> MPGPLGLLCFLALGLLGSAGPSGAAPPLCAAPCSCDGDRRVDCSGKGLTAVPEGLSAFTQALDISMNNITQLPEDAFKNFPFLEELQLAGNDLSFIHPKALSGLKELKVLTLQNNQLKTVPSEAIRGLSALQSLRLDANHITSVPEDSFEGLVQLRHLWLDDNSLTEVPVHPLSNLPTLQALTLALNKISSIPDFAFTNLSSLVVLHLHNNKIRSLSQHCFDGLDNLETLDLNYNNLGEFPQAIKALPSLKELGFHSNSISVIPDGAFDGNPLLRTIHLYDNPLSFVGNSAFHNLSDLHSLVIRGASMVQQFPNLTGTVHLESLTLTGTKISSIPNNLCQEQKMLRTLDLSYNNIRDLPSFNGCHALEEISLQRNQIYQIKEGTFQGLISLRILDLSRNLIHEIHSRAFATLGPITNLDVSFNELTSFPTEGLNGLNQLKLVGNFKLKEALAAKDFVNLRSLSVPYAYQCCAFWGCDSYANLNTEDNSLQDHSVAQEKGTADAANVTSTLENEEHSQIIIHCTPSTGAFKPCEYLLGSWMIRLTVWFIFLVALFFNLLVILTTFASCTSLPSSKLFIGLISVSNLFMGIYTGILTFLDAVSWGRFAEFGIWWETGSGCKVAGFLAVFSSESAIFLLMLATVERSLSAKDIMKNGKSNHLKQFRVAALLAFLGATVAGCFPLFHRGEYSASPLCLPFPTGETPSLGFTVTLVLLNSLAFLLMAVIYTKLYCNLEKEDLSENSQSSMIKHVAWLIFTNCIFFCPVAFFSFAPLITAISISPEIMKSVTLIFFPLPACLNPVLYVFFNPKFKEDWKLLKRRVTKKENLYFQGDYKDDDDKHHHHHHHH;> MQFRLFSFALIILNCMDYSHCQGNRWRRSKRASYVSNPICKGCLSCSKDNGCSRCQQKLFFFLRREGMRQYGECLHSCPSGYYGHRAPDMNRCARCRIENCDSCFSKDFCTKCKVGFYLHRGRCFDECPDGFAP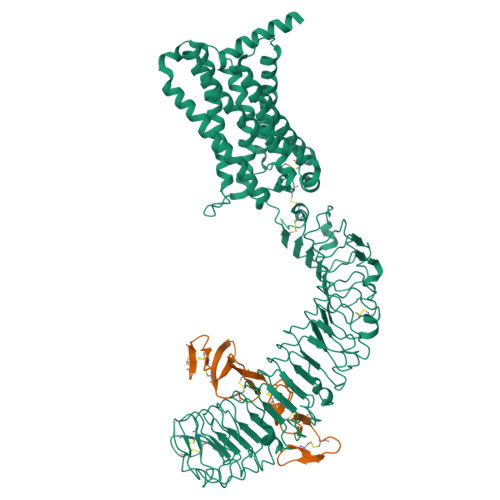LEETMECVEENLYFQGHHHHHHHHHH SisLac (also known as SisPox) is an enzyme isolated from the archaeon organism Sulfolobus islandicus, which is found in extreme environments like the Yellowstone natural park (U.S.A.) or the Mutnovksy volcano in Kamchatka (Russia). SisLac belongs to an enzyme family called Phosphotriesterase-Like Lactonase (PLL) that encompasses members from mesophilic organisms (PPH, AhlA, MCP, DrOPH) as well as thermophilic (SsoPox, SacPox, GsP, GkL) representatives. SisLac is a native lactonase that exhibits a high promiscuous phosphotriesterase activity. The catalytic mechanisms for both the lactonase and phosphotriesterase involve a nucleophilic attack by a water molecule activated by the bi-metallic center.

SisLac is homodimeric in the crystal structure with overall dimensions of the monomers of being approximately 39×48×56 Å. As for its close homolog SsoPox and related PLLs like DrOPH, GsP and GkL, SisLac is roughly globular and exhibits a (β/α)8 barrel topology. The active site consists of a binuclear center located at the C-Terminal of the barrel. Four histidines (His22, His24, His170, His199), one aspartic acid (Asp256) and a carboxylated lysine (residue 137) are coordinating the two metals. The two metal cations (possibly iron and cobalt, as seen for SsoPox and OpdA) are bridged by a water molecule that is presumed to be the catalytic nucleophile. The active site includes a long hydrophobic channel that was revealed by structural studies on SsoPox as the binding region of aliphatic chains for the AHL substrates. Indeed, SisLac’s structure is overall very similar to the structure of SsoPox (root-mean-square deviation (r.m.s.d.) for α-carbon atoms (over 314 atoms) of 0.35 Å). The dimer interface of SisLac comprises 46 residues (44 in SsoPox). The nature of this interface is mainly hydrophobic in both enzymes, but SisLac’s interface tends to be more hydrophobic (56% for SisLac, 52.6% for SsoPox), more charged (SisLac 23.91%, SsoPox 20.45%) and less polar (SisLac 32.61%, SsoPox 36.36%). Q34Y is indeed a key substitution in the interface since it consists in a “pivot” residue, i.e. a residue that contacts its equivalent in the second protein molecule while forming the dimer, and seems to be responsible for the observed dimerization shift between SisLac and SsoPox structures.

> GMRIPLVGKEPIEAEDMGFTLIHEHLRVFSEAVRYQWPHLYNEDEELRNAVNEVKRAMQFGVKTIVDPTVMGLGRDIRFMEKVVKTTGINLVAGTGIYIYVDLPFYFLNRSIDEIADLFIHDIKEGIQATSNKAGFVKIAADEPGITKDVEKVIRAAAITHKEAKVPIITHSNAHNNTGLEEQRILMEEGVDPGKILIGHLGDTDNTDYIKKIADKGSFIGLDRYGLDLFLPVDKRNETTLKLIKDGYSDRIMISHDYCCTIDWGTARPELKPKLAPRWSMALIFEDTIPFLKKNGVSEEVIDIIFKENPKKFFS> VPATRILLLVLAVIIYGTAGFHFIEGESWTVSLYWTFVTIATVGYGDYSPHTPLGMYFTCTLIVLGIGTFAVAVERLLEFL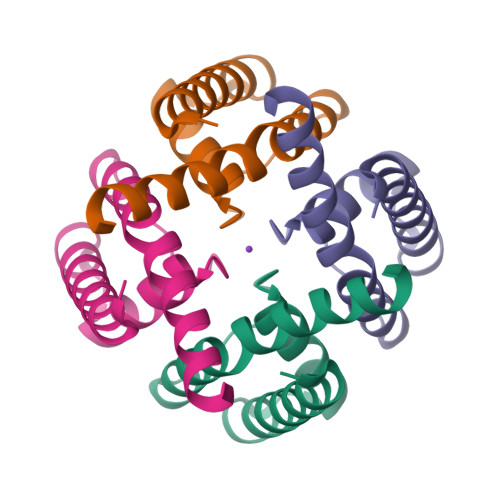IN>[4x]MERKISRIHLVSEPSITHFLQVSWEKTLESGFVITLTDGHSAWTGTVSESEISQEADDMEMEKGKYVGELRKALLSGAGPADVYTFNFSKESCYFFFEKNLK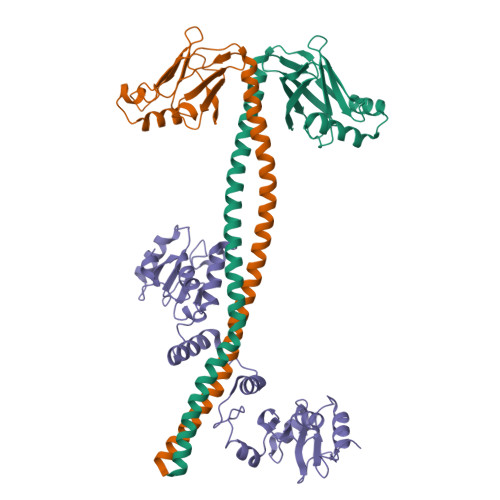DVSFRLGSFNLEKVENPAEVIRELICYCLDTTAENQAKNEHLQKENERLLRDWNDVQGRFEKCVSAKEALETDLYKRFILVLNEKKTKIRSLHNKLLNAAQ;>GAMGSKISNIFEDVEFCVMSGTDSQPKPDLENRIAEFGGYIVQNPGPDTYCVIAGSENIRVKNIILSNKHDVVKPAWLLECFKTKSFVPWQPRFMIHMCPSTKEHFAREYDCYGDSYFIDTDLNQLKEVFSGIKNSNEQTPEEMASLIADLEYRYSWDCSPLSMFRRHTVYLDSYAVINDLSTKNEGTRLAIKALELRFHGAKVVSCLAEGVSHVIIGEDHSRVADFKAFRRTFKRKFKILKESWVTDSIDKCELQEENQYLI[2x]> MKQVKAAFEANKRVYESVLLTFKGVDGYDVYNCSVPFSYKGKTHIYGRVEKRDIWAASHVRLFEETGKDEFTAVPELSWELEDPYIAKINNEMIFGGTRVRKNGNAILSYYGYFYRGTPDELTYFTRGPGCMKDIRVLQLQDGRLGVFSRPRVGRKASIGFVILNSIDELGAEVIAKAPPLDILSE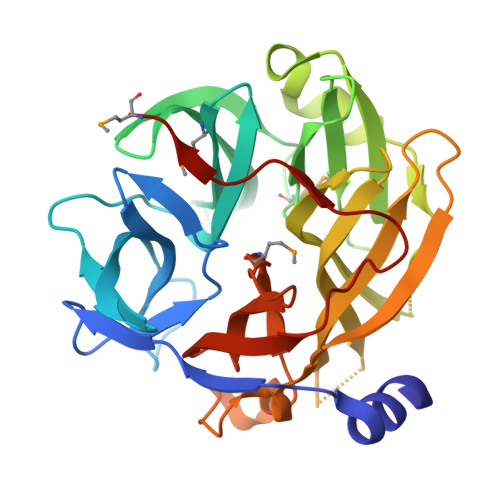NAWGGVNQAYLLSSGKVGCIGHYSYEDTNEKQQPQSVYVNYAFVLDPQSRAITGAKIIGTKSCYPPCEPKVPLLADCVFASGIVMRSDGKVDLYSGVGDSHEGRITIDYPFKGHGTIIGDLHFPMASSL>GHMGKPDISAKDLRNIMYDHLPGFGTAFHQLVQVICKLGKDS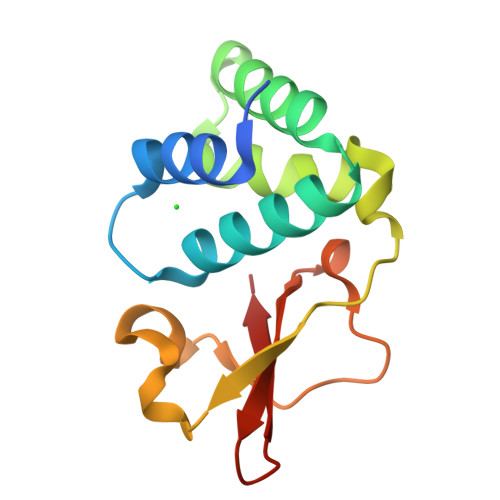NSLDIIHAEFQASLAEGDSPQCALIQITKRVPIFQDAAPPVIHIRSRGDIPRACQKSLRPVPPSPAIDAGWVCVFQLQDGKTLGLKI[2x]>MVKLFSFLLLVWVASPAFSSEFLKASGSNFYYGGQKVFLSGVNFAWRSYGSDFGNGQYASNGPALKDWINKVKASGGNTARVWVHVEGQVSPAFDSHGFVTSTDSKKTLINDLSDLLDYANGQNVFLILVLFNGALQNNSNVQNLFWDESKLNSYINNALTPMVNALKSKPSLAAWEVLNEPEGTLQPGSDQNSCYDTSTLAAQGAGWGGKKFPMKQILKTINWISSAIHNADSKALVTVGSWSELTQTDSFGYRNHYKDSCLTGAGGKSNGIINFYQMHTYSHSGKWNQNAPFKVNRWAYNVNDKPLLIGEFASVCSQNEGIQNLYKYAYNNGYNGALTWQFNSGGDCSDTYSNQMYGMQALKGQNDQSGGKGGMVSVNINHHH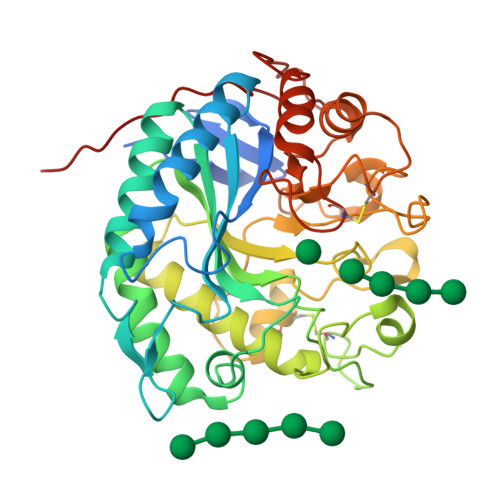HHH[2x]>MHHHHHHMTKLWAVIPAAGSGSRFSKTELKQYQYIQDATVIEHTVKRLSQLPLTGYVLAIGKQDTFASTLSFQDKHKAHFCNGGVERVHSVLNALNYLSQIADEDDWVLVHDAARPCVTFECLNTLVKNAIETNQSAILAIPVRDTLKQVNQEQQIDKTVSRELLWQAQTPQIAKIGILKKAIETALKNNLTITDEASALESIGESVQVVMGRSDNIK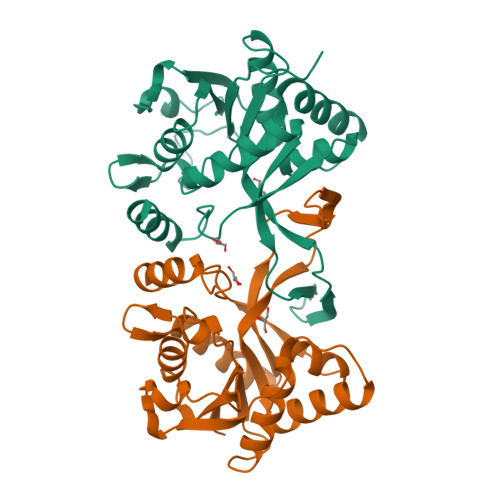ITYPDDLELARLILQSQN[2x]> GSILDGPYQ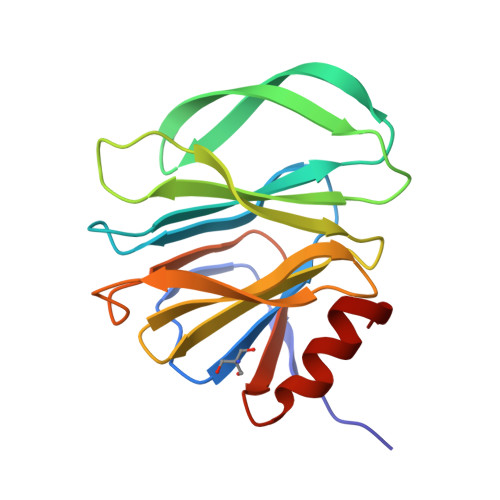PTTFKPPNDYWLLISSNTDGVVYESTNNSDFWTAVIAVEPHVSQTNRQYVLFGENKQFNVENSSDKWKFFEMFKGSSQSDFSNRRTLTSNNRLVGMLKYGGRVWTFHGETPRATTDSSNTADLNNISIIIHSEFYIIPRSQESKCNEYINNGL>SLINTKIKPFKNQAFKNGEFIEVTEKDTEGRWSVFFFYPADFTFVCPTELGDVADHYEELQKLGVD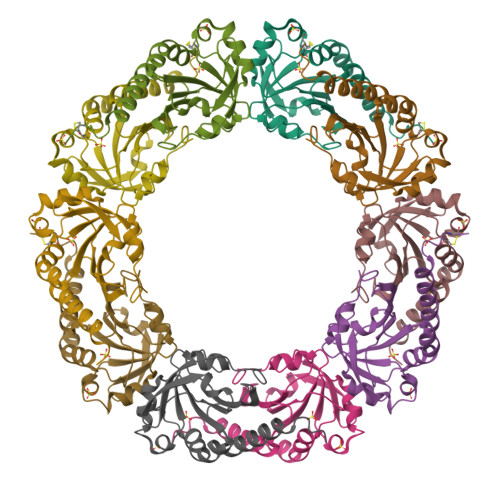VYSVSTDTHFIHKAWHSSSETIAKIKYAMIGDPTGALTRNFDNMREDEGLADRATFVVDPQGIIQAIEVTAEGIGRDASDLLRKIKAAQYVAAHPGEVCPAKWKEGEATLAPSLDLVGKI[5x]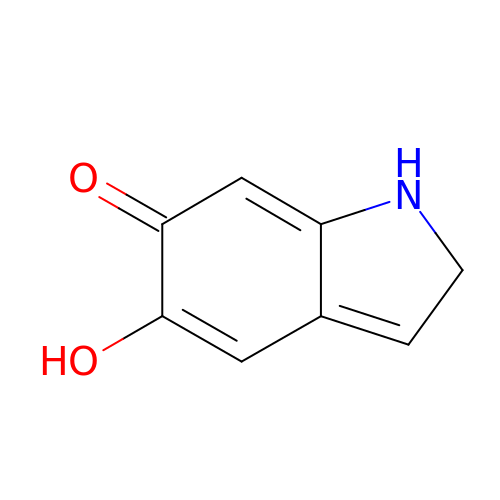5-hydroxy-1,2-dihydro-6H-indol-6-one | C8 H7 N O2 | RWEUJNADLANQCX-UHFFFAOYSA-N>MSSDYVMATKDGRMILTDGKPEIDDDTGLVSYHDQQGNAMQINRDD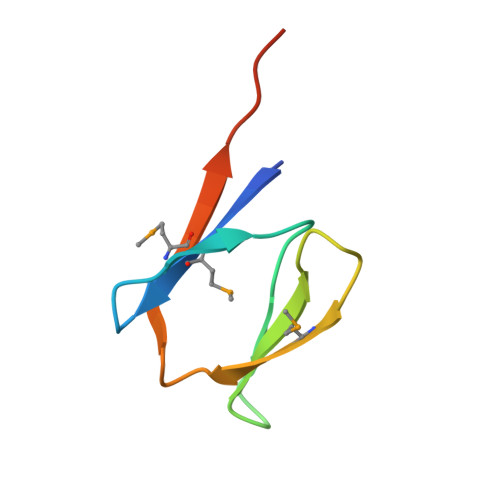VSQIIERLEHHHHHH[8x];> GGGGGGG>[2x]GELPEVETVRRELEKRIVGQKIISIEATYPRMVLTGFEQLKKELTGKTIQGISRRGKYLIFEIGDDFRLISHLRMEGKYRLATLDAPREKHDHLTMKFADGQLIYADVRKFGTWELISTDQVLPYFLKKKIGPEPTYEDFDEKLFREKLRKSTKKIK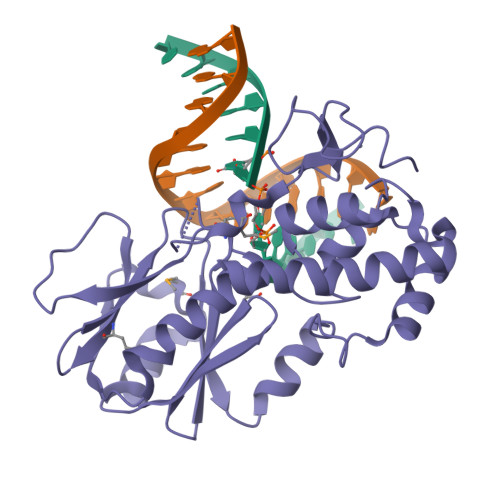PYLLEQTLVAGLGNIYVDEVLWLAKIHPEKETNQLIESSIHLLHDSIIEILQKAIKLGGSSIRTYSALGSTGKMQNELQVYGKTGEKCSRCGAEIQKIKVAGRGTHFCPVCQQK2-(cyclopentyloxy)-9-(2,6-difluorobenzyl)-N-methyl-9H-purin-6-amine 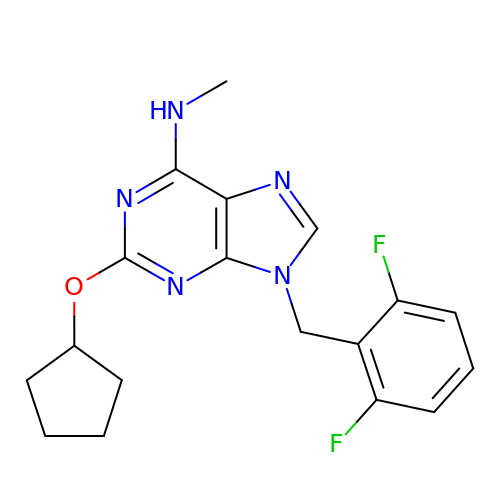| C18 H19 F2 N5 O | AWZRHMXFDZUHLF-UHFFFAOYSA-N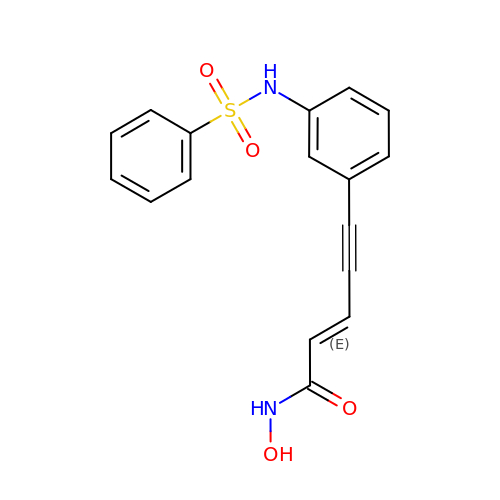Oxamflatin | C17 H14 N2 O4 S | QRPSQQUYPMFERG-LFYBBSHMSA-N In bacteria, DNA replication is initiated by the ubiquitous DnaA protein, which assembles into an oligomeric complex at the chromosome origin (oriC) that engages both double-stranded DNA (dsDNA) and single-stranded DNA (ssDNA) to promote DNA duplex opening. DnaA is a multifunctional enzyme composed of four distinct domains that act in concert during DNA replication initiation. Domain IV contains a helix-turn-helix dsDNA binding motif that specifically recognizes a 9 base pair DnaA-box (consensus 5′-TTATCCACA-3′). Domain III also contains residues that contact the phosphodiester backbone of ssDNA, along with an unidentified ssDNA binding motif that specifically recognizes the trinucleotide DnaA-trio (consensus 3′-GAT-5′).

To understand the molecular basis for specific DnaA strand separation activity, we reconstituted the BUS complex in the presence of ATP using DnaA104–446 and a tailed DNA scaffold containing a dsDNA region (DnaA-box#6 and DnaA-box#7) and a ssDNA region (DnaA-trios). Nucleoprotein complexes were crosslinked with glutaraldehyde and isolated using size exclusion chromatography before being subjected to single particle cryo-electron microscopy analysis to obtain a 3D structure of the BUS complex. Hence, the two regions of the overall map were independently determined by local refinement with a mask around the respective regions to obtain their structural information. These maps were then merged to reveal the BUS complex, composed of the spiral region at an average resolution of 3.2 Å, DNA protrusion at a resolution of 5.0 Å and the central region at 5.4 Å. The cryo-EM structure shows that DnaA assembles into a continuous oligomer that engages both dsDNA and ssDNA. DnaA1 and DnaA2 use domain IV to interact with the two available double-stranded DnaA-box motifs, engaging with DnaA-box#7 and DnaA-box#6 respectively. Remarkably, DnaA3 could also be observed to interact with dsDNA via its domain IV, where the N-terminal residues of α14 and α17 primarily engage with the backbone phosphates of the minor groove, posterior to where DnaA1 and DnaA2 interact with the DnaA-boxes. The α3 insertion into dsDNA and Lys222/Glu223 engagement with the backbone phosphate appear to distort the dsDNA structure, either of which might initiate origin unwinding. Thus, G18 and A17 are captured within a dinucleotide binding pocket created by the ISMs of adjacent DnaA protomers (DnaA1 and DnaA2). DnaA-trio#2 is engaged by DnaA2 and DnaA3, which generates an analogous nucleotide binding pocket. This pattern continues with each additional DnaA protein, resulting in a total of six DnaA-trios engaging with seven DnaA protomers to generate the domain III lattice. Inspection of the DnaA-trio interactions revealed that the two captured bases are stabilized by several hydrogen bond interactions.

>[7x]MENILDLWNQALAQIEKKLSKPSFETWMKSTKAHSLQGDTLTITAPNEFARDWLESRYLHLIADTIYELTGEELSIKFVIPQNQDVEDFMPKPQVKKAVKEDTSDFPQNMLNPKYTFDTFVIGSGNRFAHAASLAVAEAPAKAYNPLFIYGGVGLGKTHLMHAIGHYVIDHNPSAKVVYLSSEKFTNEFINSIRDNKAVDFRNRYRNVDVLLIDDIQFLAGKEQTQEEFFHTFNTLHEESKQIVISSDRPPKEIPTLEDRLRSRFEWGLITDITPPDLETRIAILRKKAKAEGLDIPNEVMLYIANQIDSNIRELEGALIRVVAYSSLINKDINADLAAEALKDIIPSSKPKVITIKEIQRVVGQQFNIKLEDFKAKKRTKSVAFPRQIAMYLSREMTDSSLPKIGEEFGGRDHTTVIHAHEKISKLLADDEQLQQHVKEIKEQLK>LVQRITIAPQGPEFSRFVMGYWRLMDWNMSARQLVSFIEEHLDLGVTTVDHADIYGGYQCEAAFGEALKLAPHLRERMEIVSKCGIATTAREENVIGHYITDRDHIIKSAEQSLINLATDHLDLLLIHRPDPLMDADEVADAFKHLHQSGKVRHFGVSNFTPAQFALLQSRLPFTLATNQVEISPVHQPLLLDGTLDQLQQLRVRPMAWSCLGGGRLFNDDYFQPLRDELAVVAEELNAGSIEQVVNAWVLRLPSQPLPIIGSGKIERVRAAVEAETLKMTRQ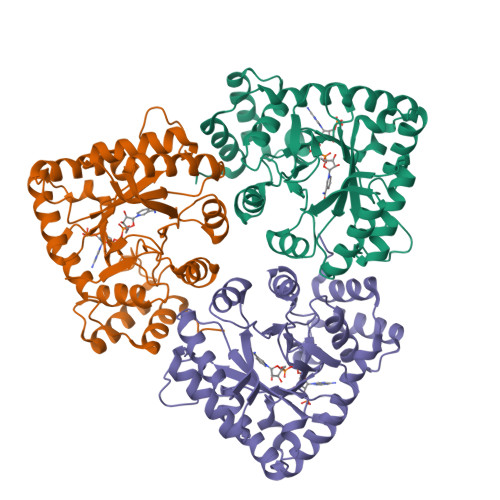QWFRIRKAALGYDVP[3x]>[8x]MAAWNYGEVAGPPTWKGVCATGKRQSPINIPLNTSAPKV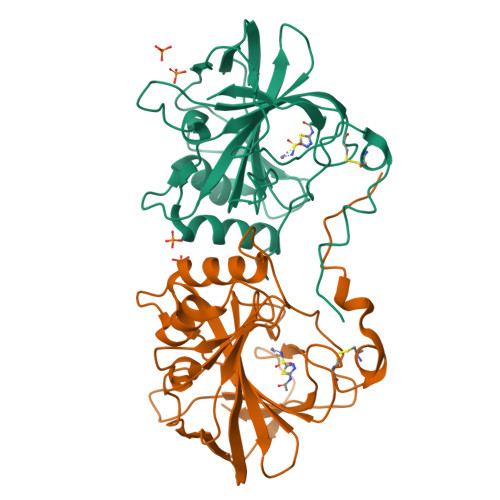DAEMGEFDFAYGSFEKCDVLNTGHGTMQVNFPAGNLAFIGNMELELLQFHFHAPSEHAMDGRRYAMEAHLVHKNKSTGNLAVLGIMLEPGGLIKNPALSTALEVAPEVPLAKKPSPKGINPVMLLPKKSKAGTRPFVHYPGSLTTPPCSEGVDWFVFMQPIKVPDSQILDFMRFVGDNKTYATNTRPLQLLNSRLVEYEL> AAESGELIGACEFMKDRLYFATLRNRPKSTINIHYFSID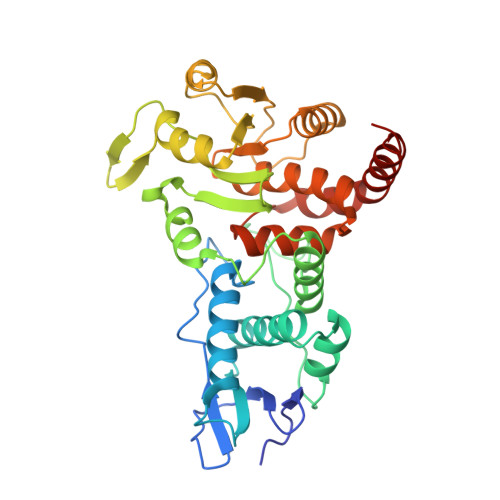EELVYENFYADFGPLNLAMVYRYCCKLNKKLKSYSLSRKKIVHYTSFDQRKRANAAFLIGAYAVIYLKKTPEEAYRALLSGSNPPYLPFRDASFGNCTYNLTVLDCLQGIRKGLQHGFFDFETFDAEEYEHYERVENGDFNWIVPGKFLAFSGPHPKSKIENGYPLHAPEAYFPYFKKNNVTTIVRLNKKIYEAKRFTDAGFEHYDLFFIDGSTPSDNIVRRFLNICENTEGAIAVHSKAGLGRTGTLIACYVMKHYRFTHAEIIAWIRICRPGSIIGPQQHFLKEKQASLWVQGDIFRSKLKNR> PISPIETVPVKLKPGMDGPKVKQWPLTEEKIKALVEICTEMEKEGKISKIGPENPYNTPVFAIKKKNSTRWRKLVDFRELNKRTQDFWEVQLGIPHPAGLKKKKSVTVLDVGDAYFSVPLDEDFRKY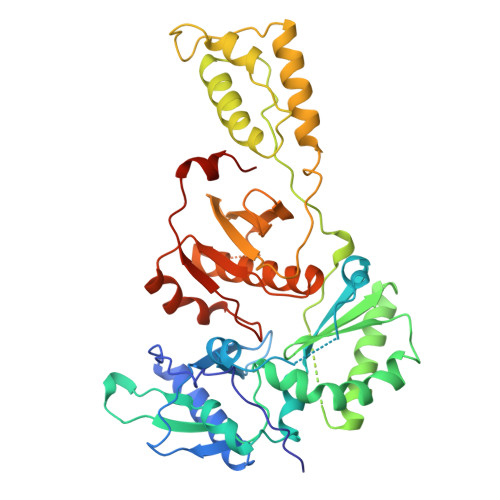TAFTIPSINNETPGIRYQYNVLPQGWKGSPAIFQSSMTKILEPFRKQNPDIVIYQYMDDLYVGSDLEIGQHRTKIEELRQHLLRWGLTTPDKKHQKEPPFLWMGYELHPDKWTVQPIVLPEKDSWTVNDIQKLVGKLNWASQIYPGIKVRQLCKLLRGTKALTEVIPLTEEAELELAENREILKEPVHGVYYDPSKDLIAEIQKQGQGQWTYQIYQEPFKNLKTGKYARMRGAHTNDVKQLTEAVQKITTESIVIWGKTPKFKLPIQKETWETWWTEYWQATWIPEWEFVNTPPLVKLWYQLEKEPIVGAETF> SGPINDTDANPRYKIPVEADFLFAYSTVPGYYSWRSPGRGSWFVQALCSILEEHGKDLEIM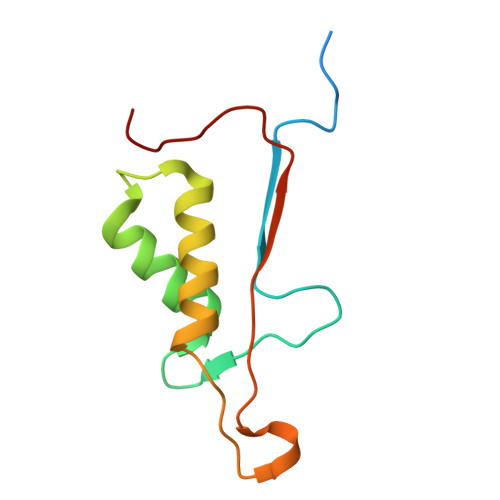QILTRVNDRVARHFESQSDDPHFHEKKQIPCVVSMLTKELYFSQ2,6-dimethoxycyclohexa-2,5-diene-1,4-dione 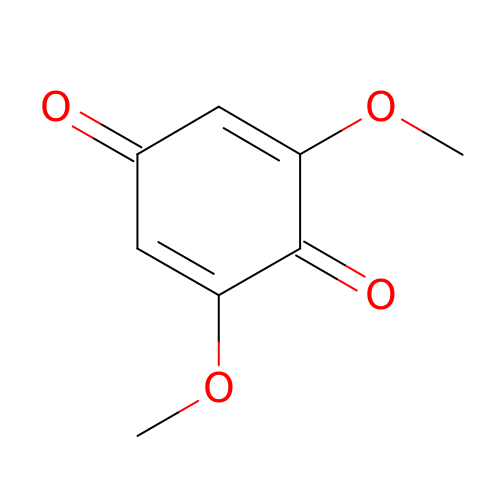| C8 H8 O4 | OLBNOBQOQZRLMP-UHFFFAOYSA-N> GSSEDKITVHFINRDGETLTTKG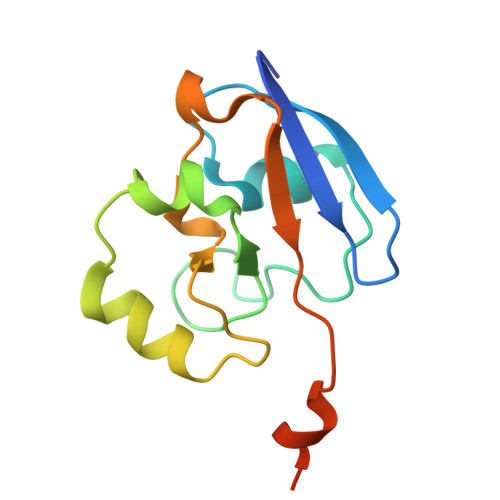KIGDSLLDVVVQNNLDIDGFGACEGTLACSTCHLIFEQHIFEKLEAITDEENDMLDLAYGLTDRSRLGCQICLTKAMDNMTVRVPDAVSDARESIDMGMNSSKIE>[4x]MTDPSKLAVAVVCSSNMN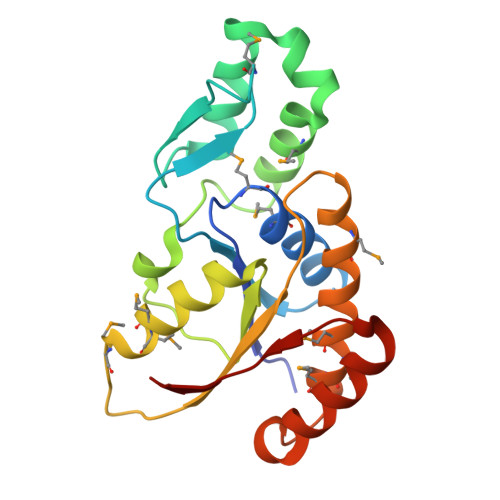RSMEAHNFLAKKGFNVRSYGTGERVKLPGMAFDKPNVYEFGTKYEDIYRDLESKDKEFYTQNGLLHMLDRNRRIKKCPERFQDTKEQFDIIVTVEERVYDLVVMHMESMESVDNRPVHVLNVDVVDNAEDALMGAFVITDMINMMAKSTDLDNDIDELIQEFEERRKRVILHSVLFY>MGSSHHHHHSSGENLYFQGHMKHGIYYSYWEHEWSAKFGPYIEKVAKLGFDIIEVAAHHINEYSDAELATIRKSAKDNGIILTAGIGPSKTKNLSSEDAAVRAAGKAFFERTLSNVAKLDIHTIGGALHSYWPIDYSQPVDKAGDYARGVEGINGIADFANDLGINLCIEVLNRFENHVLNTAAEGVAFVKDVG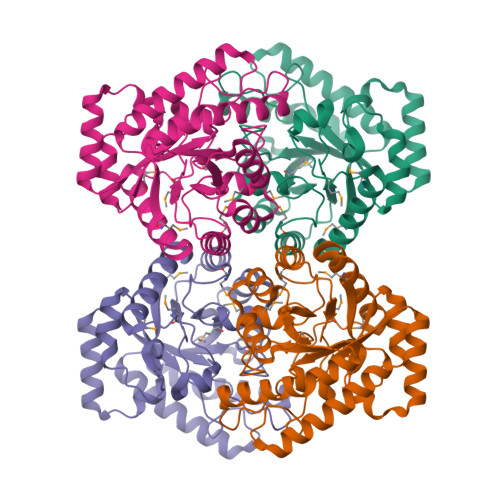KNNVKVMLDTFHMNIEEDSFGDAIRTAGPLLGHFHTGESNRRVPGKGRMPWHEIGLALRDINYTGAVIMEPFVKTGGTIGSDIKVWRDLSGGADIAKMDEDARNALAFSRFVLGG[4x]> EDVVWRWSCDNGKCVKLKNDPRSSEPALSLEACKMFCNEYGLLWPRPTGEADLGNFLSKINLNSIEVKILKKGATDDLMEAAAKRFKEQVSLAIPRGSTPKLTGKAVDVYLVNENPNEKAFS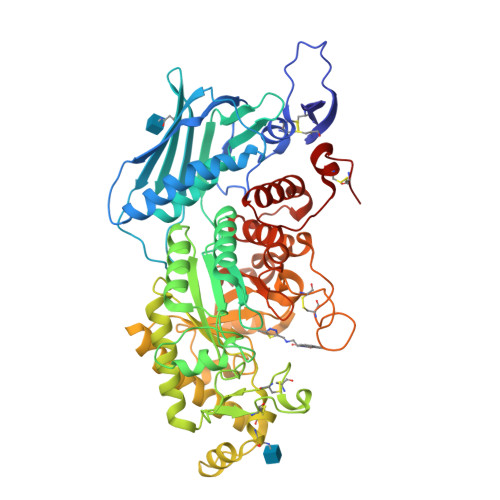LEMDESYGLRVSPSGADRVNATITANSFFGMRHGLETLSQLFVFDDIRDHLLMVRDVNISDKPVYPYRGILLDTARNYYSIESIKRTIEAMAAVKLNTLHWHITDSQSFPFVTTKRPNLYKFGALSPQKVYTKAAIREVVRFGLERGVRVLPEFDAPAHVGEGWQDTDLTVCFKAEPWKSYCVEPPCGQLNPTKDELYQYLEDIYSDMAEVFDTTDIFHMGGDEVSEACWNSSDSIQNFMMQNRWDLDKESFLKLWNYFQQKAQDKAYKAFGKKLPLILWTSTLTNYKHIDDYLNKDDYIIQVWTTGVDPQIKGLLEKGYRLIMSNYDALYFDCGYGAWVGAGNNWCSPYIGWQKVYDNSPAVIALEHRDQVLGGEAALWSEQSDTSTLDGRLWPRAAALAERLWAEPATSWQDAEYRMLHIRERFVRMGIQAESLQPEWCYQNEGYCYS>MPGSIPLIGERFPEMEVTTDHGVI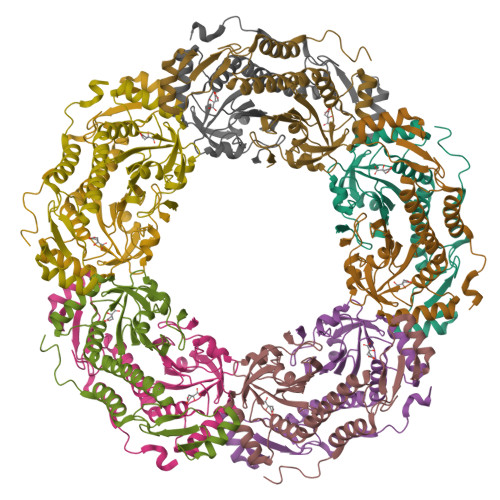KLPDHYVSQGKWFVLFSHPADATPVSTTEFVSFARRYEDFQRLGVDLIGLSVDSVFSHIKWKEWIERHIGVRIPFPIIADPQGTVARRLGLLHAESATHTVRGVFIVDARGVIRTMLYYPMELGRLVDEILRIVKALKLGDSLKRAVPADWPNNEIIGEGLIVPPPTTEDQARARMESGQYRSLDWWFSWDTPASRDDVEEARRYLRRAAEKPAKLLYEEARTHLH[10x]>HHHHHHHVTQSSSAITPGQTAELYPGDIKSVLLTAEQIQARIAELGEQIGNDYRELSATTGQDLLLITVLKGAVLFVTDLARAIPVPTQFEFMAVSSYGSSTSSSGVVRILKDLDRDIHGRDVLIVEDVVDSGLTLSWLSRNLTSRNPRSLRVCTLLRKPDA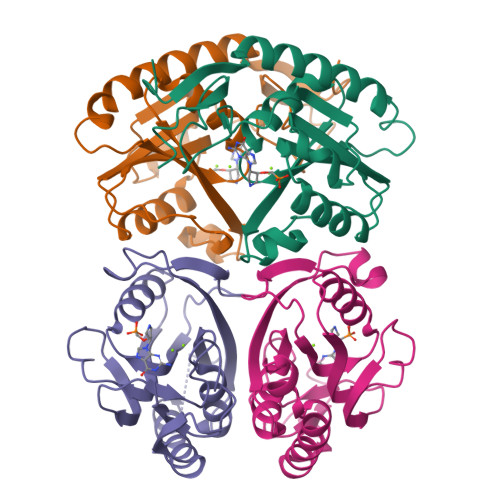VHANVEIAYVGFDIPNDFVVGYGLDYDERYRDLSYIGTLDPRVYQ[4x]> MENTLGEGSTVNASVDVDQHGNDNNSDSNANAAVAGVANTDTAGEESQQQDESLKDEATVPNTRDAESEAITVTAKQQPTMQANKLDSQETPSTEESRAQNVFGQDNEDSDNLFGETESSVSNNEANTPSIPTNPVDNENNKPAIKEDSTIQDSNGDVKNMEDVKIQKEEEPENNTVIEGVKEESQPDENTKEMDEVEEDDEDDDQPMISPDNSIFGDTKSESKQLGNTSSVANTPSEIPDAHKAEQEDIIEKTESVDKKVDSGEERNEQEREIMNDHSKSANPKKTTITRVEPETFEIPQAHEIVIPSYSKWFNLEKIHSIEVQSLPEFFTNRIPSKTPEVYMRYRNFMVNSYRLNPNEYFSVTTARRNVSGDAAALFRLHKFLTKWGLINYQVDSKLLPKNIEPPLTSQYSTRHDAPRGLFPFESYKPSVQLPDMAKLKKMMNTSDSESTLYKYLKESKRKYDEITHPPSTTDDENGDKNDNGGKMNNEVSTSTSMTGDANLLEEGETSRPLKKVKILEQIDENWSKEDLQKLLKGIQEFGADWYKVAKNVGNKSPEQCILRFLQLPIEDKFLYGDGNGKGDNDNGLGPLKYAPHLPFSKSENPVLS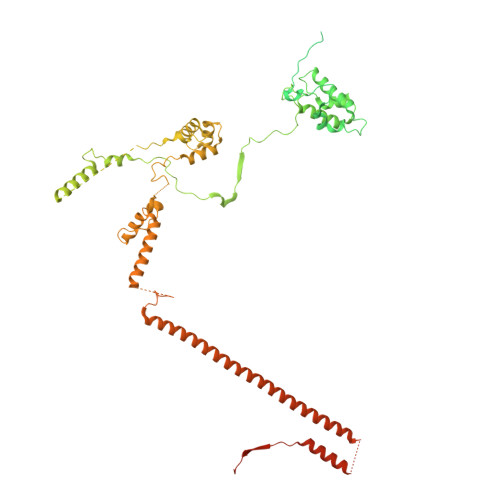TIAFLVGLVNPKTVQSMTQRAIQSAESIKSQKEEISDQKPIEHIKEGSEIAISSLGYRSHIFATNEERQMNFLTNELIRLQMEKLDAKLNHLKKLEKFMELERKTLERQQENLLIQRLNFNQNSSKIVNVLSKCLNLISDSNINNSSVAEKEEIRSQIDHFKSMLSKPETLSIGKNPFNKPNIETGENHNGQSISNENDVKPISIEAPQFYRYWSA>[2x]MEDTPLVISKQKT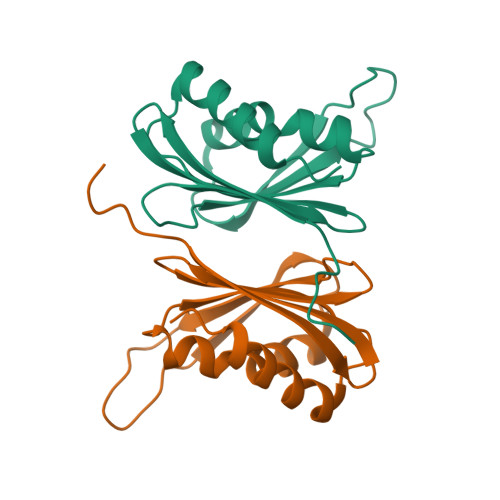EVVCGVPTQVVCTAFSSHILVVVTQFGKMGTLVSLEPSSVASDVSKPVLTTKVLLGQDEPLIHVFAKNLVAFVSQEAGNRAVLLAVAVKDKSMEGLKALREVIRVCQVW>M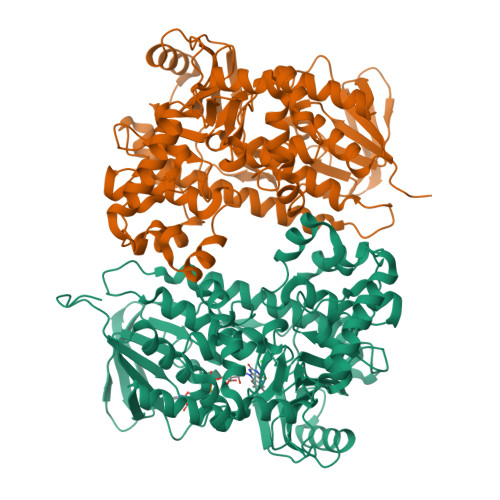TEPHRLIASNERLGTAPEAPADDDPGAIRTVGVIGGGTAGYLTALALKAKRPWLDVALVESADIPIIGVGEATVSYMVMFLHHYLGIDPAEFYQHVRPTWKLGIRFEWGSRPEGFVAPFDWGTGSVGLVGSLRETGNVNEATLQAMLMTEDRVPVYRGEGGHVSLMKYLPFAYHMDNARLVRYLTELAARRGVRHVDATVAEVRLDGPDHVGGLITTDGRRLHYDFYVDCTGFRSLLLEKALGIPFESYASSLFTDAAVTGTLAHGGHLKPYTTATTMNAGWCWTIPTPESDHLGYVFSSAAIDPDDAAAEMARRFPGVTREALVRFRSGRHREAWRGNVMAVGNSYAFVEPLESSGLLMIATAVQILVSLLPSSRRDPLPSDAANQALAHRWDAIRWFLSIHYRFNGRLDTPFWKEARAETDISGIEPLLRLFAAGAPLTGRDSFTRYLADGAAPLFYGLEGVDTLLLGQEVPARLLPPREPPEQWRARAAAARSLASRGLRQSEALDAYAADPCLNAELLSDSDSWAGERVAVRAGLR[4x]> GPMTTTERPDLAWLDEVTMTQLERNPYEVYERLRAEAPLAFV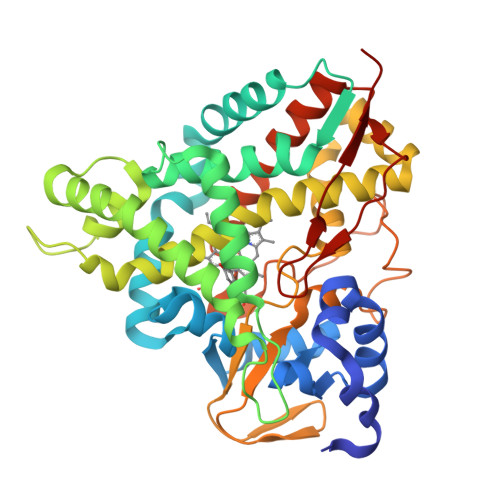PVLGSYVASTAEVCREVATSPDFEAVITPAGGRTFGHPAIIGVNGDIHADLRSMVEPALQPAEVDRWIDDLVRPIARRYLERFENDGHAELVAQYCEPVSVRSLGDLLGLQEVDSDKLREWFAKLNRSFTNAAVDENGEFANPEGFAEGDQAKAEIRAVVDPLIDKWIEHPDDSAISHWLHDGMPPGQTRDREYIYPTIYVYLLGAMQEPGHGMASTLVGLFSRPEQLEEVVDDPTLIPRAIAEGLRWTSPIWSASARISTKPVTIAGVDLPAGTPVMLSYGSANHDTGKYEAPSQYDLHRPPLPHLAFGAGNHACAGIYFANHVMRIALEELFEAIPNLERDTREGVEFWGWGFRGPTSLHVTWEV> GNNIEVIKMVEVKLENLTKRFGNFTAVNKLNLTIKDGEFLVLLGPSGCGKTTTLRMIAGLEEPTEGRIYFGDRDVTYLPPKDRNISMVFQSYAVWPHMTVYENIAFPLKIKKFPKDEIDKRVRWAAELLQIEELLNRYPAQLSGGQRQRVAVARAIVVEPDVLLMDEPLSNLDAKLRVAMRAEIKKLQQKLKVTTIYVTHDQVEAMTMGDRIAVMNRGQLLQIGSPTEVYLRPN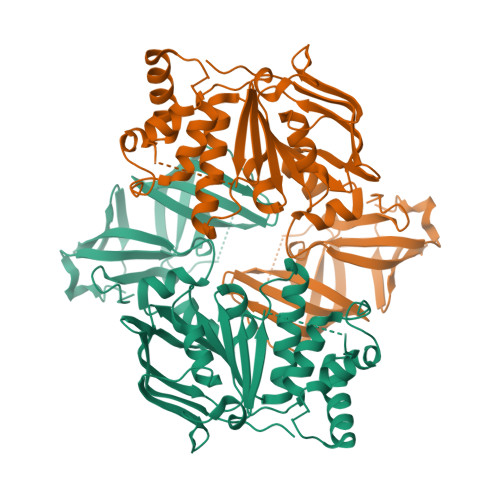SVFVATFIGAPEMNILEVSVGDGYLEGRGFRIELPQDLMDLLKDYVGKTVLFGIRPEHMTVEGVSELAHMKRTARLIGKVDFVEALGTDTILHVKFGDELVKVKLPGHIPIEPGREVKVIMDLDMIHVFDKDTEKAIV> MENLNMDLLYMAAAVMMGLAAIGAAIGIGILGGKFLEGAARQPDLIPLLRTQFFIVMGLVDAIPMIAVG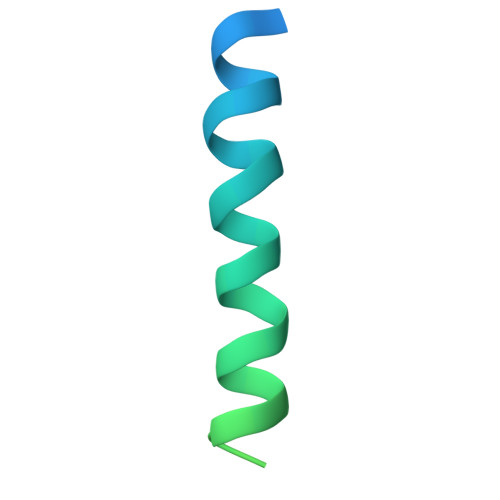LGLYVMFAVA>MTQTYNADAIEVLTGLEPVRRRPGMYTDTTRPNHLGQEVIDNSVDEALAGHAKRVDVILHADQSLEVIDDGRGMPVDIHPEEGVPAVELILCRLHAGGKFSNKNYQFSGGLHGVGISVVNALSKRVEVNVRRDGQVYNIAFENGEKVQDLQVVGTCGKRNTGTSVHFWPDETFFDSPRFSVSRLTHVLKAKAVLCPGVEITFKDEINNTEQRWCYQDGLNDYLAEAVNGLPTLPEKPFIGNFAGDTEAVDWALLW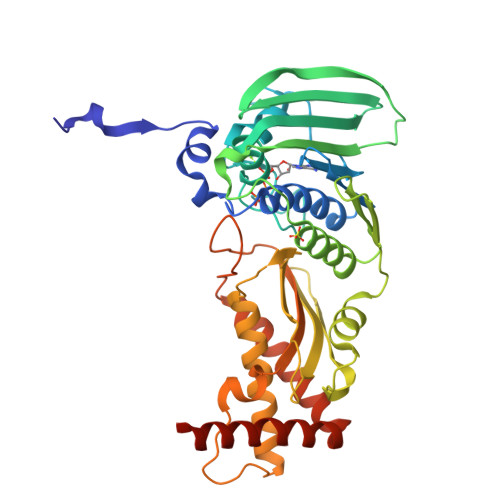LPEGGELLTESYVNLIPTMQGGTHVNGLRQGLLDAMREFCEYRNILPRGVKLSAEDIWDRCAYVLSVKMQDPQFAGQTKERLSSRQCAAFVSGVVKDAFILWLNQNVQAAELLAEMAISSAQRRMRAAKKVVRKK[2x]> MTLAISVGVLMAGFVFLVLQRGMVRVILGFILLSHAAHLTLMAAGGASRREAPLVSDPDPALTSDGLPQAFVLTAIVIAFAITIYLLVLAVIGGDDDDTDIGDLDPLDLLPE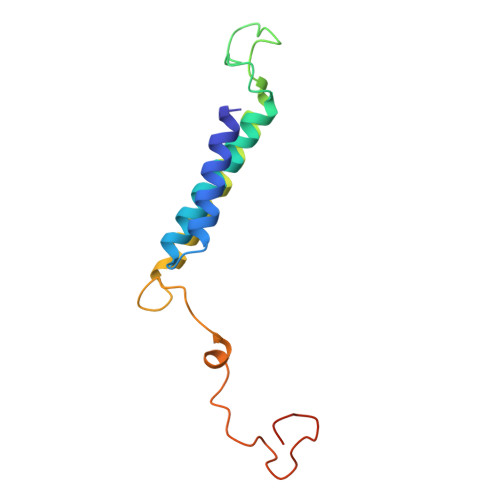TPGGAHPEDPEPDEPSTHDAEGVHR>[4x]NAMVVTLDGEILQPGMPLLHADDLAAVRGDGVFETLLVRDGRACLVEAHLQRLTQSARLMDLPEPDLPRWRRAVEVATQRWVAST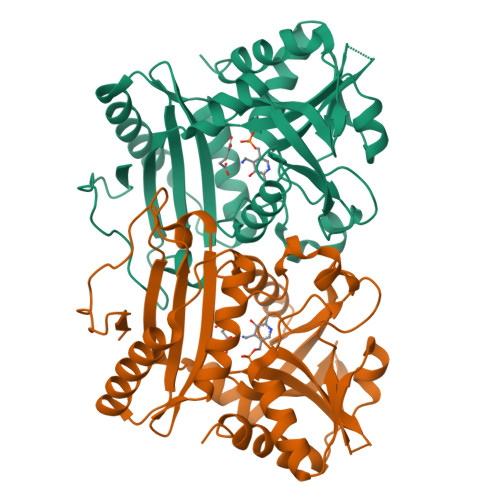ADEGALRLIYSRGREGGSAPTAYVMVSPVPARVIGARRDGVSAITLDRGLPADGGDAMPWLIASAKTLSYAVNMAVLRHAARQGAGDVIFVSTDGYVLEGPRSTVVIATDGDQGGGNPCLLTPPPWYPILRGTTQQALFEVARAKGYDCDYRALRVADLFDSQGIWLVSSMTLAARVHTLDGRRLPRTPIAEVFAELVDAAIVSDR> MSSAEEKLFMKALKEKFEESPEEKYTKFYIFGGWKQSERKKEFKEWADKIVEERGVPHYNPDIGVPLGQRKLMSYQVSGTDVFVEGDDLTFVNNAAMQQMWDDIRRTVIVGMDTAHRVLERRLGKEVTPETINEYMETLNHALPGGAVVQEHMVEIHPGLTWDCYAKIITGDLELADEIDDKFLIDIEKLFPEEQAEQLIKAIGNRTYQVCRMPTIVGHVCDGATMYRWAAMQIAMSFICAYKIAAGEAAVSDFAFASKHAEVINMGEMLPARRARGENEPGGVPFGVLADCVQTMRKYPDDPAKVALEVIAAGAMLYDQIWLGSYMSGGVGFTQYATAV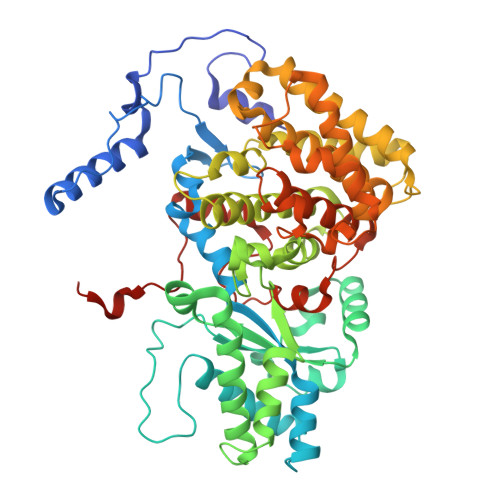YPDNILDDYVYYGLEYVEDKYGIAEAEPSMDVVKDVATEVTLYGLEQYERYPAAMETHFGGSQRAAVCAAAAGCSTAFATGHAQAGLNGWYLSQILHKEGQGRLGFYGYALQDQCGAANSLSVRSDEGLPLELRGPNYPNYAMNVGHLGEYAGIVQAAHAARGDAFCVHPVIKVAFADENLVFDFTEPRKEFAKGALREFEPAGERDLIVPAE> MSSYESIDFFTDPSLIPDPHPYFDYLRSQSPVLRLPQYGVVAVTGYEEATAVYKDTDSFSNCVALGGPFPPLPFAPNGDDVNAQIDAHREQFPMYEHMVTMDPPEHSRARSILSRLLTP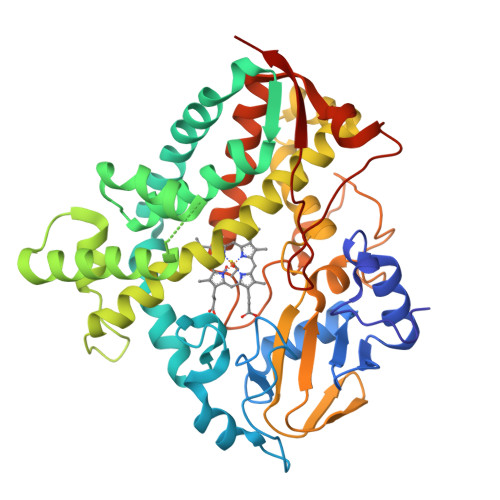SRLKQNEEFMWRLADRQLDEFLGAGECEFISEYAKPFATLVIADLLGVPEDDRKDFRVVLGADRMGRVGALDHESVGVNPLQWLDDKFSAYIEDRRRQPRNDVLTALATATYPDGSTPEVIDVVRSATFLFAAGQETTAKLLTAAMRVLGDRPDIQRRLRENRSLIPNFIEESLRMDSPVKSDSRLARKRTTVGGLDIAAGTVVMVLPGAANRDPRRFEDPHEFRLDRPNVREHMAFARGVHSCPGGPLARVEGRVSLERILDRMLDIAINEDRHGPADDRRYTYEPTYILRGLTELHITFTPAG>IFPKQYPIINFTTADATVESYTNFIRAVRSHLTTGADVRHEIPVLPNRVGLPISQRFILVELSNHAELSVTLALDVTNAYVVGCRAGNSAYFFHPDNQEDAEAITHLFTDVQNSFTFAFGGNYDRLEQLGGLRENIELGTGPLEDAISALYYYSTCGTQIPTLARSFMVCIQMISEAARFQYIEGEMRTRIRYNRRSAPDPSVITLENSWGRLSTAIQESNQGAFASPIQLQRRNGSKFNVYDVSI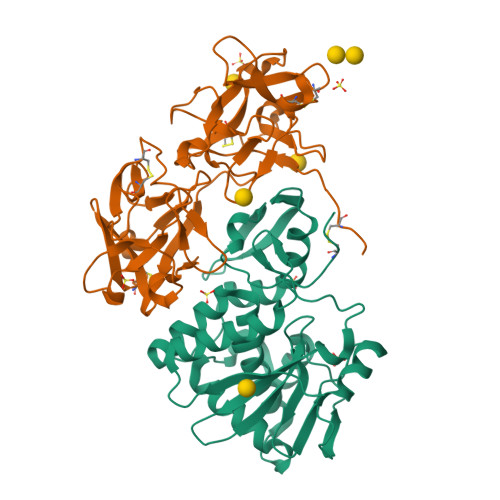LIPIIALMVYRCAPPP[2x];>ADVCMDPEPIVRIVGRNGLCVDVTGEEFFDGNPIQLWPCKSNTDWNQLWTLRKDSTIRSNGKCLTISKSSPRQQVVIYNCSTATVGATRWQIWDNRTIINPRSGLVLAATSGNSGTKLTVQTNIYAVSQGWLPTNNTQPFVTTIVGLYGMCLQANSGKVWLEDCTSEKAEQQWALYADGSIRPQQNRDNCLTTDANIKGTVVKILSCGPASSGQRWMFKNDGTILNLYNGLVLDVRRSDPSLKQIIVHPFHGNLNQIWLPLF[2x]> MSREVKRIGDGLFVTIEPANDVR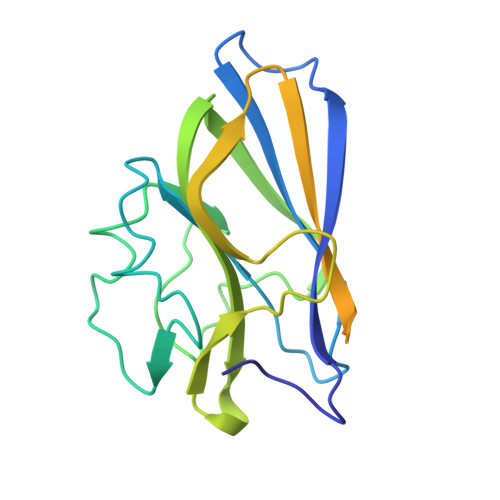ANEAKVVLAADNVWGDNTGYQFLLDADHNTFGSVIPATGPLFTGTASSDLYSANFEYLIPANADPVVTTQNIIVTGQGEVVIPGGVYDYCITNPEPASGKMWIAGDGGNQPARYDDFTFEAGKKYTFTMRRAGMGDGTDMEVEDDSPASYTYTVYRDGTKIKEGLTETTYRDAGLSAQSHEYCVEVKYTAGVSPKVC>[16x]GPPSRVIHIRKL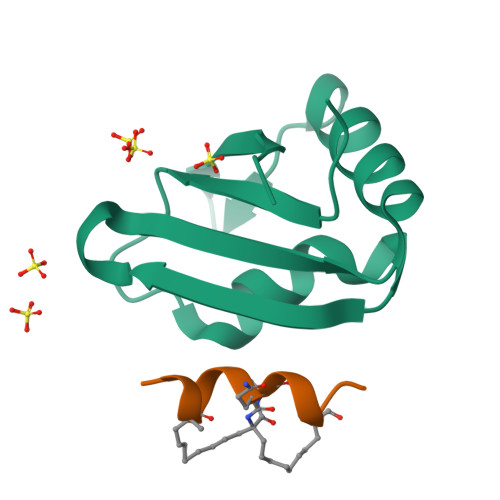PIDVTEGEVISLGLPFGKVTNLLMLKGKNQAFIEMNTEEAANTMVNYYTSVTPVLRGQPIYIQFSNHKELKTDS;>NQLRAQXALQXVN[16x]>MNTLDTLPVHPRTGLRAIGMGKRGPIWPVMGASDDHKDDAPTLTYSQARNRADEVHARMEQIAELDKPTDEENEEFRALGAEFDSLVNHMSRLERAAELARVRSTHEQIGKPQSGGQRRMRVEAGSSQGGRGDYDRDAILEPDSIEDCRFRDPWNLSEMRTFGRDAEEVKGELRARALSAIEKMQGASDNVRAAATHIIERFDDEDSTLARQCLATSSPAYLRAWSKMARNPHAAILTEEEKRAINEVRAMGLTKADGGYLVPFQLDPTVIITSNGSLNDIRRFARQVVATGDVWHGVSSAAVQWSWDAEFEEVSDDSPEFGQPEIPVKKAQGFVPISIEALQDEANVTETVALLFAEGKDELEAVTL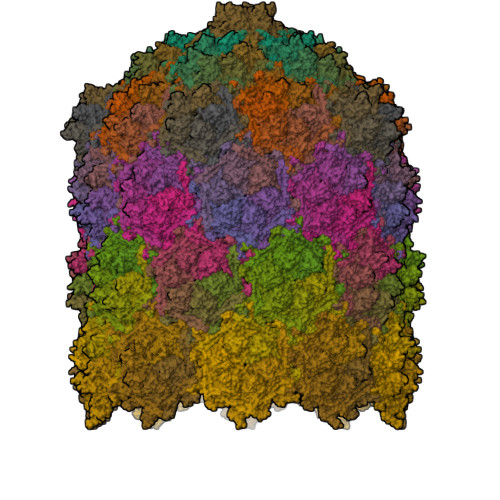TTGTGQGNQPTGIVTALAGTAAEIAPVTAETFALADVYAVYEQLAARHRRQGAWLANNLIYNKIRQFDTQGGAGLWTTIGNGEPSQLLGRPVGEAEAMDANWNTSASADNFVLLYGNFQNYVIADRIGMTVEFIPHLFGTNRRPNGSRGWFAYYRMGADVVNPNAFRLLNVETAS[54x]>ANVRLQHHHHHHHLEASDQRGYKPEDVAFDESFFSFGGHVGTSVEYEDKVTRGFNNTDKKEKTITNEVFNFFYNNPQWNFMGFYSFKIENREQKEPGYYENEDGIKQLFSLNKGHDLGNGWATGLIYELEYTRSKVYSPDVSGLRKNLAEHSIRPYLTYWNNDYNMGFYSNLEYLLSKEDRNAWGKRQEQGYSALFKPYKRFGNWEVGVEFYYQIKTNDEKQPDGTINEKSDFNERYIEPIVQYSFDDAGTLYTRVRVGKNETKNTDRSGGGNAGINYFKDIRKATVGYEQSIGESWVAKAEYEYANEVEKKSRLSG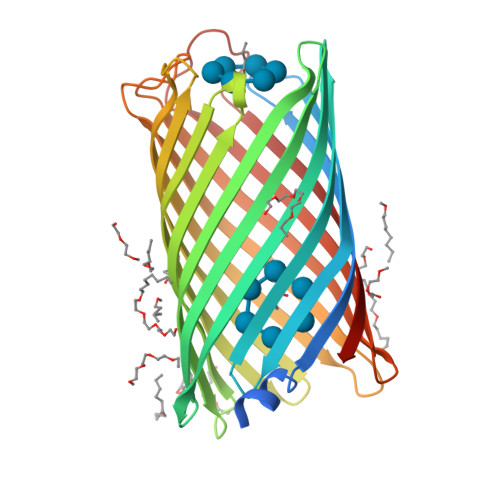WEARNKSELTQHTFYAQALYRF[2x]> MGINGQQYYIDPTTGQPRKNFLLQSGNNWIYFDSDTGVGTNALELQFAKGTVSSNEQYRNGNAAYSYDDKSIENVNGYLTADTWYRPKQILKDGTTWTDSKETDMRPILMVWWPNTLTQAYYLNYMKQHGNLLPSALPFFNADADPAELNHYSEIVQQNIEKRI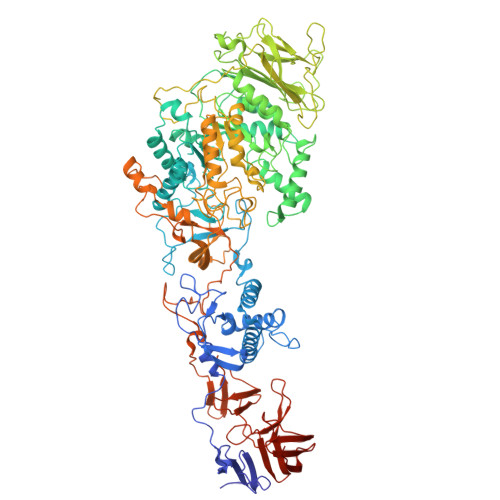SETGNTDWLRTLMHDFVTNNPMWNKDSENVNFSGIQFQGGFLKYENSDLTPYANSDYRLLGRMPINIKDQTYRGQEFLLANDIDNSNPVVQAEQLNWLYYLLNFGTITANNDQANFDSVRVDAPDNIDADLMNIAQDYFNAAYGMDSDAVSNKHINILEDWNHADPEYFNKIGNPQLTMDDTIKNSLNHGLSDATNRWGLDAIVHQSLADRENNSTENVVIPNYSFVRAHDNNSQDQIQNAIRDVTGKDYHTFTFEDEQKGIDAYIQDQNSTVKKYNLYNIPASYAILLTNKDTIPRVYYGDLYTDGGQYMEHQTRYYDTLTNLLKSRVKYVAGGQSMQTMSVGGNNNILTSVRYGKGAMTATDTGTDETRTQGIGVVVSNTPNLKLGANDKVVLHMGAAHKNQQYRAAVLTTTDGVINYTSDQGAPVAMTDENGDLYLSSHNLVVNGKEEADTAVQGYANPDVSGYLAVWVPVGASDNQDARTAPSTEKNSGNSAYRTNAAFDSNVIFEAFSNFVYTPTKESERANVRIAQNADFFASLGFTSFEMAPQYNSSKDRTFLDSTIDNGYAFTDRYDLGMSEPNKYGTDEDLRNAIQALHKAGLQVMADWVPDQIYNLPGKEVATVTRVDDRGNVWKDAIINNNLYVVNTIGGGEYQKKYGGAFLDKLQKLYPEIFTKKQVSTGVAIDPSQKITEWSAKYFNGTNILHRGSGYVLKADGGQYYNLGTTTKQFLPIQLTGEKKQGNEGFVKGNDGNYYFYDLAGNMVKNTFIEDSVGNWYFFDQDGKMVENKHFVDVDSYGEKGTYFFLKNGVSFRGGLVQTDNGTYYFDNYGKMVRNQTINAGAMIYTLDENGKLIKASYNSDAEYPTSTDVGKMLDQNKLHHHHHH> MGAGREVSVSLDGVRDKNLMQLKILNTVLFPVRYNDKYYADAIAAGEFTKLAYYNDICVGAIACRLEKKESGAMRVYIMTLGV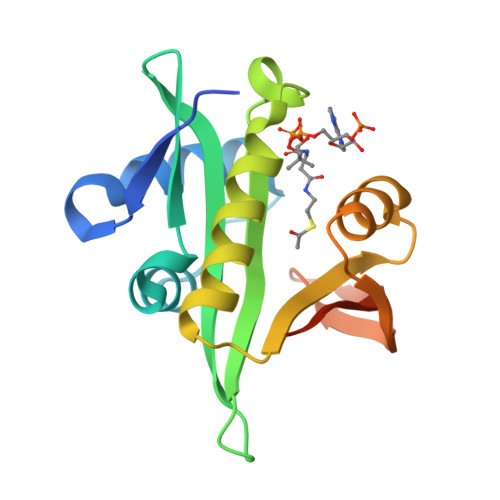LAPYRGIGIGSNLLNHVLDMCSKQNMCEIYLHVQTNNEDAIKFYKKFGFEITDTIQNYYINIEPRDCYVVSKSFAQSEANKHHHHHH>MACTWPAWEQFKKDYISQEGRVIDPSDARKITTSEGQSYGMFSALAANDR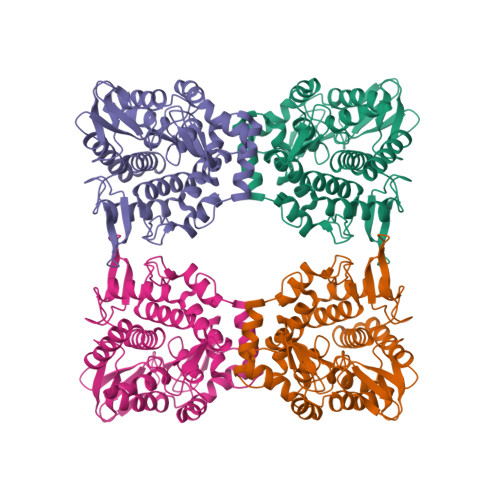AAFDNILDWTQNNLAQGSLKERLPAWLWGKKENSKWEVLDSNSASDGDVWMAWSLLEAGRLWKEQRYTDIGSALLKRIAREEVVTVPGLGSMLLPGKVGFAEDNSWRFNPSYLPPTLAQYFTRFGAPWTTLRETNQRLLLETAPKGFSPDWVRYEKDKGWQLKAEKTLISSYDAIRVYMWVGMMPDSDPQKARMLNRFKPMATFTEKNGYPPEKVDVATGKAQGKGPVGFSAAMLPFLQNRDAQAVQRQRVADNFPGSDAYYNYVLTLFGQGWDQHRFRFSTKGELLPDWGQECANSHLEHHHHHH[4x]(2~{S})-1-(2-methoxyethoxy)propan-2-amine | C6 H15 N O2 | 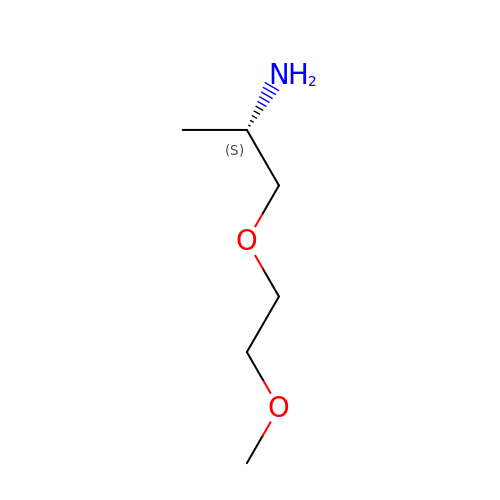CMXIILNXYHCYPP-LURJTMIESA-N> SGKNP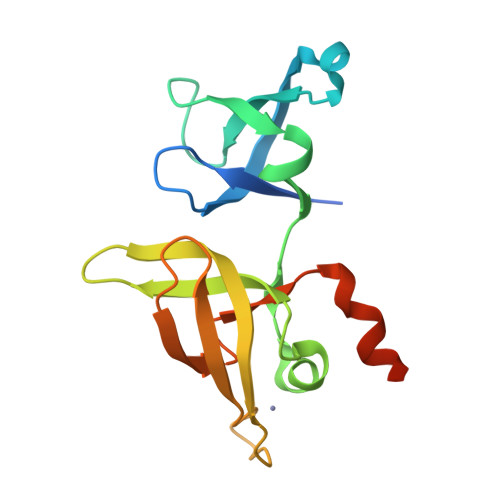VESVSVEFEAKSARDGAWYDVAAFLSHRLFESGDPEVRVRFSGFGAEEDEWINVRKCVRQRSLPCEATECVAVLPGDLILCFQEGKDQALYYDAHVLDAQRRRHDVRGCRCRFLVRYDHDSSEEIVPLRKVCRRPETDYRLQILHAARAAATN>GMDLHSLLELGTKPTAPHVRNKKVILFDTNHQVSICNQIIDAINSGIDLGDLLEGGLLTLCVEHYYNSDKDKFNTSPIAKYLRDAGYEFDVIKNADATRFLDVIPNEPHYSPLILALKTLESTESQRGRIGLFLSFCSLFLPKLVVGDRASIEKALRQVTVHQEQGIVTYPNHWLTTGHMKVIFGILRSSFILKFVLIHQGVNLVTGHDAYDSIISNSVGQTRFSGLLIVKTVLEFILQKTDSGVTLHPLVRTSKVKNEVASFKQALSNLARHGEYAPFARVLNLSGINNLEHGLYPQLSAIALGVATAHGSTLAGVNVGEQYQQLREAAHDAEVKLQRRHEHQEIQAIAEDDEERKILEQFHLQKTEITHSQTLAVLSQKREKLARLAAEIENNIVEDQGFKQSQNRVSQSFLNDPTPVEVTVQARPMNRVEHHHHHHHH[3x]

Marburg virus (MARV) is an enveloped, non-segmented, single-stranded negative-sense RNA (ssRNA -) virus that belongs to the Filoviridae family, order Mononegavirales, and causes lethal disease in humans and non-human primates. Therefore, research aimed at investigating the MARV proteome to validate antiviral targets and to decipher the structural aspects of its mechanism of infection stands as the utmost priority. Among the seven proteins encoded by the MARV genome, the nucleoprotein (NP) exerts its fundamental role in encapsidating ssRNA into a helical ribonucleoprotein (RNP) complex, which in turn serves as scaffold for nucleocapsid formation, viral RNA transcription, and replication. We determined by cryogenic electron microscopy (cryo-EM) the MARV helical ribonucleoprotein (RNP) complex structure in single-layered conformation, which differs from the previously reported structure of a double-layered helix.

To fill this knowledge gap, in this work we report the detailed structure of MARV RNP complex in a more compact single-layer conformation, reconstituted in vitro by assembling recombinant NP onto synthetic ssRNA, imaged by cryo-EM and determined by single particle analysis (SPA) helical reconstruction. In agreement with the results from 2D classification and 3D reconstruction, atomic modeling of the MARV RNP complex structure describes a single-stranded, left-handed (h -) hollow helix with inner and outer diameters of 164 Å and 285 Å, respectively. Each helix turn is completed by ~ 25 NP subunits, and repeats with a pitch of about 70 Å. Indeed, our structure revealed that an intra-chain, non-canonical parallel coiled-coil is formed in the MARV NPcore between the helices α15 and α16, stabilizing the C-lobe in an orientation that favors both clamping of the ssRNA by helix η6 and NPcore interaction with adjacent protomers via helix α16. Interactions between NPcore protomers and ssRNA are only intra-strand ones, established in such a way that any given hexameric RNAn is wrapped by the corresponding NPn protomer, but also interacts with the adjacent ones NPn+1 and NPn −1. Overall, binding of each NPcore protomer to a 6 nt-long tract of the 18 nt ssRNA in the asymmetric minimal unit of the single-layered MARV RNP complex follows the same modality, and involves the same set of highly conserved amino acid residues, as in the double-layered structure, with any hexameric RNAn tract being clamped by the NPn η6 and α17 C-lobe helices to accommodate, twisted in a “three-bases-in, three-bases-out” conformation, into the groove beneath the NPn N-lobe. Moreover, substantiating the rationale for a sequence-independent RNA-binding fashion, most interactions are electrostatics in character and established between the ssRNA phosphate backbone and basic amino acids such as Lys142, Lys153, Arg156 and Lys230, which were previously proven by mutagenesis as important - to various extent – for both RNP complex assembly and ssRNA synthesis.> MGSSHHHHHHSSGENLYFQGSNSEGDYQLVQHEVLCSMTNTYEVLEFLGRGTFGQVVKCWKRGTNEIVAIKILKNHPSYARQGQIEVSILARLSTESADDYNFVRAYECFQHKNHTCLVFEMLEQNLYDFLKQNKFSPLPLKYIRPVLQQVATALMKLKSLGLIHADLKPENIMLVDPSRQPYRVKVIDFGSASHVSKAVCSTYLQSR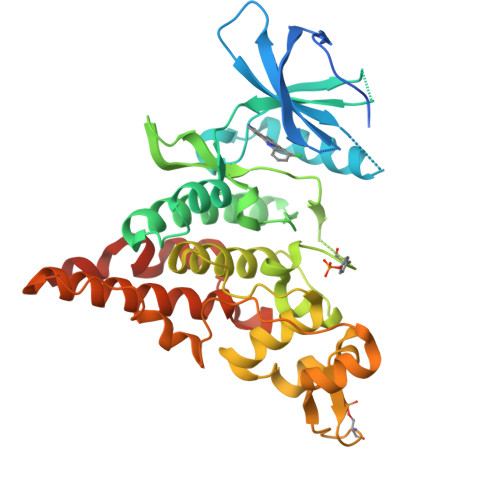YYRAPEIILGLPFCEAIDMWSLGCVIAELFLGWPLYPGASEYDQIRYISQTQGLPAEYLLSAGTKTTRFFNRDTDSPYPLWRLKTPDDHEAETGIKSKEARKYIFNCLDDMAQVNMTTDLEGSDMLVEKADRREFIDLLKKMLTIDADKRITPIETLNHPFVTMTHLLDFPHSTHVKSCFQN N-{[4-(4-phenyl-1,3-thiazol-2-yl)tetrahydro-2H-pyran-4-yl]methyl}-3-[5-(trifluoromethyl)-1,2,4-oxadiazol-3-yl]benzamide 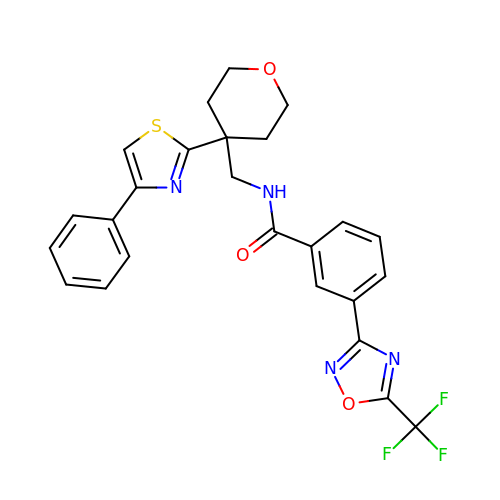| C25 H21 F3 N4 O3 S | HORXBWNTEDOVKN-UHFFFAOYSA-N(1R,2S,3S,4R,5R,9S,11S,12S,14R)-7-amino-2,4,12-trihydroxy-2-(hydroxymethyl)-10,13,15-trioxa-6,8-diazapentacyclo[7.4.1.1~3,12~.0~5,11~.0~5,14~]pentadec-7-en-8-ium 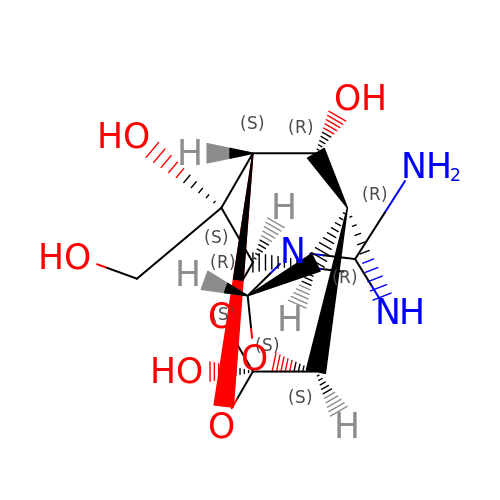(non-preferred name) | C11 H15 N3 O7 | STNXQECXKDMLJK-LQRXLWILSA-N The multi-subunit Type III-A CRISPR-Cas effector complex (Csm) exemplifies this principle and is in addition regulated by cellular metabolites such as divalent metals and ATP. Recognition of the foreign or cognate target RNA (CTR) triggers its single-stranded deoxyribonuclease (DNase) and cyclic oligoadenylate (cOA) synthesis activities. The same activities remain dormant in the presence of the self or non-cognate target RNA (NTR) that differs from CTR only in its 3′-protospacer flanking sequence (3′-PFS). The single-stranded DNase (ssDNase) and the cOA synthesis activities reside within the Csm1 subunit and the RNase activity resides within Csm317–19.

Two distinct CTR-bound structures were resolved from two major classes that have 1123344151crRNA1Target1 (CTR-43) and 1122334151crRNA1Target1 (CTR-32) stoichiometry, respectively, where each number corresponds to a numbered Csm protein. Interestingly, unlike previously determined thermophilic Csm structures that prefer assemblies with fewer numbers of Csm3 and Csm224,25, LlCsm prefers the longer CTR-43. In contrast, though no ATP was used in formation of CTR-bound LlCsm, we observed 3′-PFS traversing through Csm1.

> MDKINLVCGSLLHNIGKIIYRGTSERAKHSKLGGDFIKSFEQFRNTELTDCIRYHHAQEITSVKSNKEKNSLFYITYIADNISSGMDRRKDLEEGAEGFNWDKKVALGSVFNVLNEKEKGRQNYSYPFVARTRIKEEPLNFPTATQNQYTTSYYDGLITDMKTILQRLKPDKEHINSLLQMMESLWSYVPSSTDKNQLVDISLYDHSRTTAAIASAIYDYFQAENITDYQKELFDYNATEFYDKNAFLMMNFDMSGVQNFIYNISGSKALKSLRARSFYLDMLLEYISDNLLEKLELSRANILYVGGGHAYLLLANTNKTKAILSDFEHDLKTWFLDKFKIDLYVAMAYTEVSANDLMNHNGHYRDIYRRLSQKTSAKKANRYTAEEILNLNHQGTENARECRECKRSDLLIEEDDICEICDSLQKVSRDLTRENIFVIANEGVLDMPFGKKMSALSYSQADKLKKSNAEVQIYAKNISEIGQNLMTRIDMGDYTYRSDFHEMLEEVEVGINRLGVLRADVDNLGQAFINGIPDDYLSISRTATFSRAMSRFFKNYLNQLLAEKSYKINVIYAGGDDLFMIGAWQDILDFSIVLKQKFADFTQNKLSISAGIGMFREKYPVARMASLTGDLEDAAKDYKPDERAVQATKNAVTLFDATNVFSWDTLENDIFVKLDAITKNFEKLDETGKAFIYRLIDLLRGVNENQQINIARLAYTLSRMEEKIGKTFAQELYNWANADRKTLIMALEIYILKTRE;> MKIIKLYFESPVHFGEKRLSESKITFSADTLFSALMIEAVGLGKEDEFYQLASNNLVKFSDAFPFIDQYYYIPKPMFNLKLEKEDENPSKAFKKLLYVPIDSLEDYLSGGLDAYFERESFNLGKLALSEKVQQHDFKDSEPYNVGTFTFKENTGLYVLIEQTHPLLEELLENLQYSGIGGKRNSGYGKFKFEILEDSDIEDLFSAKGNRKILLSGALPKDAELEQALKNASYLLERRGGFVQSDTYATNLVKKQDLYVFKSGSTFENSFDGDIYQVGKKGNHPVYKYAKSFFLEVS;>[2x]TELKIGNEKVNSTNFGDFAEKAIRGINHKPFVNSKGGEQKITTSKIRGILELVNKVYNRVINTNDVELSENILADIAYIKVKIAYESGREPVVKDFIQRTAFTAAITDVMNQRTRESFLLFARYVESLIAYFKFYGGKD;>[3x]MKLVIEGTIVLKTGMHIGGSSDFSAIGAVASPVVRDTLTRLPLIPGSSLKGKMRYLLAKELNNGILLNEPNNDQDEILRLFGSSEKDKIRRARLKFNDIKLSNLAELETFNVSSTEVKFENTINRKTAVANPRQIERVIAGSKFDFEIFYNLDDIKEVEKDFENIKQGFDLLEFDYLGGHGTRGSGRIAFENLSVITAVGNFEKINTLNEILGA;> MKKTYRVTLTALGPIFIGGGEKLKKYEYIFDKQKKVAHMIDHTKFTKYLLEKNLLDDFTSRVNSHFDLYDYLVNKKGIVFMPLVKYSVPVAQFRTEVKNRFGKPISSPPMNDLNTFVKDAFGRPYIPGSSLKGALRTAILNDLKEDTKENEVFAHLQVSDSETIDLENLKVYQKVDYSKTAKPLPLYRECLKPNTEITFTVSFDDEYLTLKKIQNALHKTYQHYYIKWLKGGKVGETLIKGVYDSHADELKKNTFALDQPSQNQGEIIYIGGGAGFVSKTLHYKSKNRDQARNDSFDILKQLFRTTYSKMRSVPDNVPVALKLAVETKTFNGRVTGKHYLEMGKARIKLEEL> MGGGVSVELPKRDPPPGVPTDEMLLNVDKMHDVIAPAKLLEYVH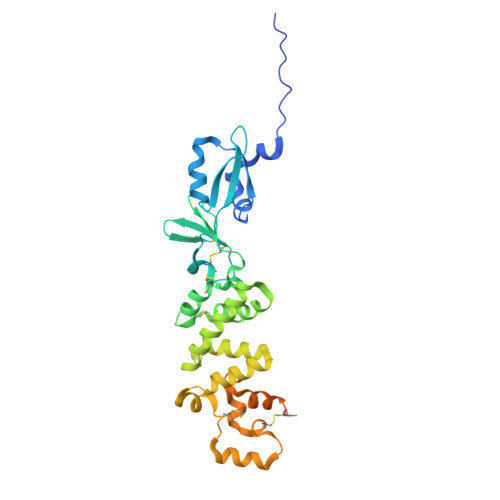IGPLAKDKEDKVKKRYPEFRLVNTGPGGLSALLRQSYNGTAPNCCRTFNRTHYWKKDGKISDKYEEGAVLESCWPDVHDTGKCDVDLFDWCQGDTFDRNICHQWIGSAFNRSNRTVEGQQSLINLYNKMQTLCSKDASVPICESFLHHLRAHNTEDSKEMIDYILRQQSADFKQKYMRCSYPTRDKLEESLKYAEPRECWDPECSNANVNFLLTRNYNNLGLCNIVRCNTSVNNLQMDKTSSLRLSCGLSNSDRFSTVPVNRAKVVQHNIKHSFDWSHPQFEK> ALSPPRRKSFKKWTPPRSPFNLVQEILFHD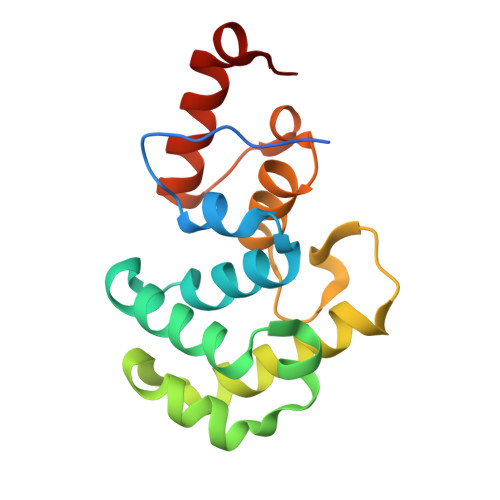PWKLLIATIFLNRTSGKMAIPVLWEFLEKYPSAEVARAADWRDVSELLKPLGLYDLRAKTIIKFSDEYLTKQWRYPIELHGIGKYGNDSYRIFCVNEWKQVHPEDHKLNKYHDWLWENHEKLSLS The heterodinuclear Mn/Fe cofactor is found in the R2 subunits of subclass Ic ribonucleotide reductases (denoted as R2c) as well as a related group of proteins known as R2-like ligand-binding oxidases (R2lox). Although the physiological function of R2lox proteins is not known, the cofactor catalyzes formation of a tyrosine–valine ether cross-link in the protein scaffold. Two proteins from this group have been characterized to date, homologs from Mycobacterium tuberculosis and Geobacillus kaustophilus. Both contain the ether cross-link, and both co-purify from heterologous expression hosts with a long-chain fatty acid ligand bound in a hydrophobic channel leading from the protein surface to the active site, hence the name ligand-binding oxidase. The two metal ions are bound next to each other in octahedral geometry by two histidines and four glutamates, with the manganese ion occupying the N-terminal metal-binding site 1.

Crystal structures were obtained of all three R2lox point mutants in the non-activated reduced and the oxidized resting state by soaking apo-protein crystals with MnII and FeII under anoxic or aerobic conditions, respectively. In contrast, the bulky isoleucine side chain in V72I-R2lox has a larger effect on Y162 than on the metal-coordinating residues. It seems to have displaced the Y162 side chain, particularly in the reduced state. Aside from these two residues, however, the structures of V72I-R2lox are practically identical to the wild-type structures in both redox states. Judging from the crystal structures, it appears likely that the barrier for photoactivation is lowered due to steric hindrance caused by the bulky isoleucine sidechain, making coordination of Fe2 a more favorable position for Y162 than in the wild-type.

>MAHHHHHHVDDDDKMVHHDGFQTVKATIDWEHPMFKLYEKAKRNGKWNPADIDFSQDQKDFASLTSEEKISALPLVAGFSAGEEAITLDILPMAHALARQGRLEDVLFLTTFMHDEAKHVEMFSRWQQAVGIGQMDLSVFHNDHYKRIFYEALPEAMNRLYADDSPEAVIRAATVYNMIVEGTLAESGYYTFRQIYKKAGLFPGLLQGIDYLNMDEGRHIQFGIYTIQRIVNEDERYYELFIRYMDELWPHVIGYVDYLTELGKRQQQLARTYALEIDYDLLRHYVIKQFNLRKKQISRTKRVDVVEGLEKTAAES[2x]A family of four soluble lectins has been identified in B. cenocepacia, all of them containing at least one domain with strong sequence similarity with LecB (PA-IIL) from Pseudomonas aeruginosa. BC2L-C has an N-terminal region of 155 amino acids (the TNF-α-like lectin), a 28-aa linker region, and a 115-aa C-terminal region. Since the isolated BC2L-C-nt domain binds strongly to fucose but not to mannose and galactose, BC2L-C is therefore a novel type of lectin consisting of independent fucose and mannose-binding domains. To our knowledge, BC2L-C is the first protein identified harbouring two different lectin domains with distinct specificity, for which we refer to it to as a “superlectin”.

The C-terminal domain has sequence similarity with two-calcium bacterial lectins such as LecB/PA-IIL from P. aeruginosa (43% identity) and related ones. BC2L-C-ct bound to Man and α-methyl-mannoside (αMeMan) with a strong affinity in the micromolar range but with a stoichiometry close to 0.5, indicating that only one binding site per dimer is accessible. BC2L-C-ct is dimeric in solution with a molecular mass of 22±1 kDa whereas BC2L-C-nt is trimeric with a molecular mass of 41±1 kDa (the expected monomeric masses are 12.4 kDa and 19.3 kDa, respectively). The dimeric association displays close similarity to the lectin BC2L-A, described previously. In contrast to other crystal structures in this family, no electron density for calcium ions and monosaccharide (d-mannose) was found in the final model, presumably due to the presence of citric acid in the crystallization buffer. Without the stabilizing effect of the two calcium ions in the binding site, the acidic amino acids that mediate their binding appear to point in all directions. A sulphate ion was observed close to one of the two binding sites, establishing hydrogen bonds with Gln241, His177 and two bridging water molecules. The main difference with the mannose-binding site of RS-IIL is the presence of His177 (Asn in all other lectins). In the absence of calcium, this histidine interacts with one sulphate ion but also modifies the conformation of the C-terminus of the other chain. Since the C-terminal carboxyl group has an essential role in binding mannose and calcium in all the other similar lectins, the putative destabilizing role of His177 could account for the observed non-even stoichiometry of the dimer.

>[2x]MERDGTFNLPPHIKFGVTALTHAANDQTIDIYIDDDPKPAATFKGAGAQDQNLGTKVLDSGNGRVRVIVMANGRPSRLGSRQVDIFKKSYFGIIGSEDGADDDYNDGIVFLNWPLG N-(2-chloro-6-fluorobenzyl)-1-methyl-N-{[3'-(methylsulfonyl)biphenyl-4-yl]methyl}-1H-imidazole-4-sulfonamide 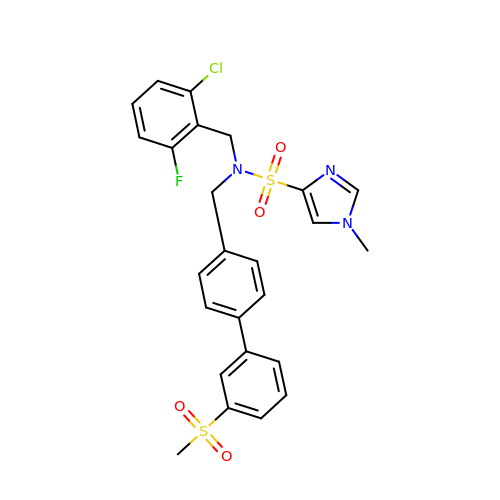| C25 H23 Cl F N3 O4 S2 | AYVVQXQFVKEXMX-UHFFFAOYSA-N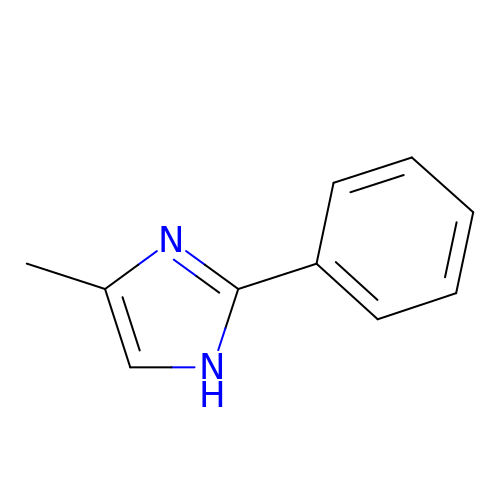4-methyl-2-phenyl-1H-imidazole | C10 H10 N2 | TYOXIFXYEIILLY-UHFFFAOYSA-N As exemplified by isoniazid, which targets the enoylreductase in mycolic acid biosynthesis, mycocerosic acid synthase (MAS) offers a potential drug target by producing part of phthiocerol dimycocerosate (PDIM), a key component of the cell envelope. MAS, a fully reducing iterative type I polyketide synthase (PKS), is composed of six domains that together catalyze the elongation of n-C6-C20 fatty acids to prepare mycocerosic acid. Using a combination of dual covalent crosslinking and cryo-EM analyses, we elucidate the structure of mycocerosic acid synthase from Mycobacterium tuberculosis trapped in two distinct catalytic states during its iterative cycle. These structures reveal domain architecture of the acyl carrier protein mediating condensation and dehydration through dual site-selective crosslinking of the acyl carrier protein with the ketosynthase and dehydratase domains.

We obtained a density map with 3.87 Å resolution from samples of the ACPs = KSs ( = indicates crosslink) dual crosslinked protein, complex A, including all domains KS, AT, DH, ΨKR, ER, KR, and ACP. Both ACPs are crosslinked at the homodimeric KS domains, linking Ser2060 in ACP with Cys177 in KS with the C16 acyl tail bound within the canonical KS substrate pocket. The crosslinkers tethered on the ACPA and ACPB through a 4’-phosphopantetheine (PPant) arm are well resolved within the KS • KS’ binding tunnels, each making a covalent linkage at the active site Cys residues (Cys177 in KS and KS’). The full MAS structure adopts a homodimeric architecture, comprising two catalytic chambers (chambers 1 and 2). The dimerization interface is comprised of the KS • KS’ (2566 Å2), DHA • DHB (429 Å2), and ERA • ERB (1165 Å2) domains. Supported by partial density, a 14 residue flexible KR-ACP linker (L5) allows the ACP to travel between the domains of each of the catalytic chambers of MAS. Due to the flexibility offered by the linker-based architecture, complex A is not perfectly symmetrical. Distances between the active site residues Tyr1912 (KR) and Ser623 (AT), as well as Tyr1912 (KR) and Ser2060 (ACP), are 78.1 Å and 71.9 Å, respectively, in protomer 1, compared with 72.4 Å and 69.6 Å inter-residue distances in protomer 2, revealing a significant in-plane tilting movement of the modifying compartment that pivots at the KS • KS’ core. The AT domain in complex A is in the apo form (without substrate in the active site), consisting of an α/β-hydrolase and ferredoxin subdomains, sharing a similar fold with other type I and type II systems. The absence of observed “turnstile closed” conformations in MAS complexes A and B implies that iterative type I PKSs utilize a different mechanism to prevent premature reloading of the KS domain.

>[2x]MESRVTPVAVIGMGCRLPGGINSPDKLWESLLRGDDLVTEIPPDRWDADDYYDPEPGVPGRSVSRWGGFLDDVAGFDAEFFGISEREATSIDPQQRLLLETSWEAIEHAGLDPASLAGSSTAVFTGLTHEDYLVLTTTAGGLASPYVVTGLNNSVASGRIAHTLGLHGPAMTFDTACSSGLMAVHLACRSLHDGEADLALAGGCAVLLEPHASVAASAQGMLSSTGRCHSFDADADGFVRSEGCAMVLLKRLPDALRDGNRIFAVVRGTATNQDGRTETLTMPSEDAQVAVYRAALAAAGVQPETVGVVEAHGTGTPIGDPIEYRSLARVYGAGTPCALGSAKSNMGHSTASAGTVGLIKAILSLRHGVVPPLLHFNRLPDELSDVETGLFVPQAVTPWPNGNDHTPKRVAVSSFGMSGTNVHAIVEEAPAEASAPESSPGDAEVGPRLFMLSSTSSDALRQTARQLATWVEEHQDCVAASDLAYTLARGRAHRPVRTAVVAANLPELVEGLREVADGDALYDAAVGHGDRGPVWVFSGQGSQWAAMGTQLLASEPVFAATIAKLEPVIAAESGFSVTEAITAQQTVTGIDKVQPAVFAVQVALAATMEQTYGVRPGAVVGHSMGESAAAVVAGALSLEDAARVICRRSKLMTRIAGAGAMGSVELPAKQVNSELMARGIDDVVVSVVASPQSTVIGGTSDTVRDLIARWEQRDVMAREVAVDVASHSPQVDPILDDLAAALADIAPMTPKVPYYSATLFDPREQPVCDGAYWVDNLRNTVQFAAAVQAAMEDGYRVFAELSPHPLLTHAVEQTGRSLDMSVAALAGMRREQPLPHGLRGLLTELHRAGAALDYSALYPAGRLVDAPLPAWTHARLFIDDDGQEQRAQGACTITVHPLLGSHVRLTEEPERHVWQGDVGTSVLSWLSDHQVHNVAALPGAAYCEMALAAAAEVFGEAAEVRDITFEQMLLLDEQTPIDAVASIDAPGVVNFTVETNRDGETTRHATAALRAAEDDCPPPGYDITALLQAHPHAVNGTAMRESFAERGVTLGAAFGGLTTAHTAEAGAATVLAEVALPASIRFQQGAYRIHPALLDACFQSVGAGVQAGTATGGLLLPLGVRSLRAYGPTRNARYCYTRLTKAFNDGTRGGEADLDVLDQHGTVLLAVRGLRMGTGTSERDERDRLVSERLLTLGWQQRALPEVGDGEAGSWLLIDTSNAVDTPDMLASTLTDALKSHGPQGTECASLSWSVQDTPPNDQAGLEKLGSQLRGRDGVVIVYGPRVGDPDEHSLLAGREQVRHLVRITRELAEFEGELPRLFVVTRQAQIVKPHDSGERANLEQAGLRGLLRVISSEHPMLRTTLIDVDEHTDVERVAQQLLSGSEEDETAWRNGDWYVARLTPSPLGHEERRTAVLDPDHDGMRVQVRRPGDLQTLEFVASDRVPPGPGQIEVAVSMSSINFADVLIAFGRFPIIDDREPQLGMDFVGVVTAVGEGVTGHQVGDRVGGFSEGGCWRTFLTCDANLAVTLPPGLTDEQAITAATAHATAWYGLNDLAQIKAGDKVLIHSATGGVGQAAISIARAKGAEIFATAGNPAKRAMLRDMGVEHVYDSRSVEFAEQIRRDTDGYGVDIVLNSLTGAAQRAGLELLAFGGRFVEIGKADVYGNTRLGLFPFRRGLTFYYLDLALMSVTQPDRVRELLATVFKLTADGVLTAPQCTHYPLAEAADAIRAMSNAEHTGKLVLDVPRSGRRSVAVTPEQAPLYRRDGSYIITGGLGGLGLFFASKLAAAGCGRIVLTARSQPNPKARQTIEGLRAAGADIVVECGNIAEPDTADRLVSAATATGLPLRGVLHSAAVVEDATLTNITDELIDRDWSPKVFGSWNLHRATLGQPLDWFCLFSSGAALLGSPGQGAYAAANSWVDVFAHWRRAQGLPVSAIAWGAWGEVGRATFLAEGGEIMITPEEGAYAFETLVRHDRAYSGYIPILGAPWLADLVRRSPWGEMFASTGQRSRGPSKFRMELLSLPQDEWAGRLRRLLVEQASVILRRTIDADRSFIEYGLDSLGMLEMRTHVETETGIRLTPKVIATNNTARALAQYLADTLAEEQAAAPAASKLAAALEHHHHHH ICAM-5, initially called telencephalin, is an integral type I transmembrane glycoprotein of ∼150 kDa that is expressed exclusively in telencephalic neurons. It has nine immunoglobulin superfamily (IgSF) domains, with a total of 832 amino acids in the extracellular region, a single transmembrane segment and a 64-residue cytoplasmic domain. In addition to integrin recognition shared with the other ICAMs, ICAM-5 has unique characteristics within the subfamily, as it mediates homophilic adhesion interactions that promote neurite development. The crystal structure of the four most N-terminal glycosylated domains (D1–D4) of ICAM-5 was determined in three different space groups and the D1–D5 fragment was modelled.

In interface B, D1 interacted similarly with D4 in the P21 and R3 crystal structures. Interface B includes positively and negatively charged surfaces in D1 and D4, respectively, and four salt bridges. In the P21 crystal structure, we identified two similar antiparallel arrangements of symmetry-related ICAM-5 molecules with contacts between the N-terminal and C-terminal portions. The head (D1–D2) and tail (D3–D4) of one IC5-4D molecule contacted two distinct symmetry-related partners; each contact buried 500–600 Å2 of surface area and included charged residues in all four interacting domains. In addition, three acidic residues in D3–D4 formed salt bridges with the D1–D2 arginines. The second type of crystal contact buried a smaller surface area (500 Å2) and included no glycans (interface D); a single IC5-4D molecule also interacted with two symmetry-related molecules that buried about 1000 Å2 of its surface. In contrast, in the monoclinic P21 crystals the IC5-4D molecules assemble with an antiparallel orientation and the crystal lattice generates two similar antiparallel trans/trans zippers that resemble the assemblies described for other homophilic cell adhesion structures. This type of zipper could represent of ICAM-5 homophilic cell adhesion complexes. One of the crystal lattices has a molecular assembly that could represent the homophilic ICAM-5 cell adhesion complex in neurons.

> EPFWADLQPRVAFVERGGSLWLNCSTNCPRPERGGLETSLRRNGTQRGLRWLARQLVDIREPETQPVCFFRCARRTLQARGLIRTFQRPDRVELMPLPPWQPVGENFTLSCRVPGAGPRASLTLTLLRGAQELIRRSFAGEPPRARGAVLTATVLARREDHGANFSCRAELDLRPHGLGLFENSSAPRELRTFSLSPDAPRLAAPRLLEVGSERPVSCTLDGLFPASEARVYLALGDQNLSPDVTLEGDAFVATATATASAEQEGARQLVCNVTLGGENRETRENVTIYSFPAPLLTLSEPSVSEGQMVTVTCAAGAQALVTLEGVPAAVPGQPAQLQLNATENDDRRSFFCDATLDVDGETLIKNRSAELRVLYAPR> GAMGMSYAYLFK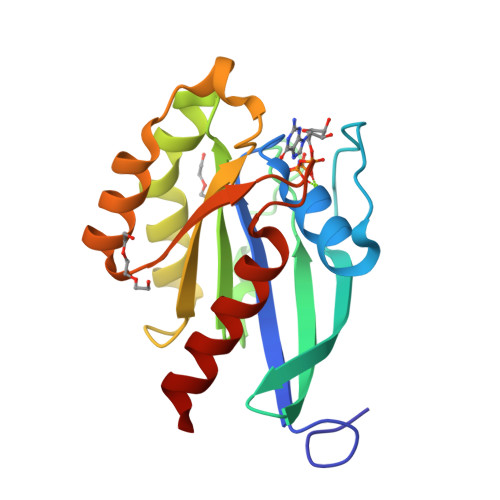YIIIGDTGVGKSCLLLQFTDKRFQPVHDLTIGVEFGARMITIDGKQIKLQIWDTAGLEAFRSITRSYYRGAAGALLVYDITRRETFNHLTTWLEDARQHSNSNMVIMLIGNKSDLDSRREVKKEEGEAFAREHGLVFMETSARTAANVEEAFINTAKEIYEKIQ> PQYEY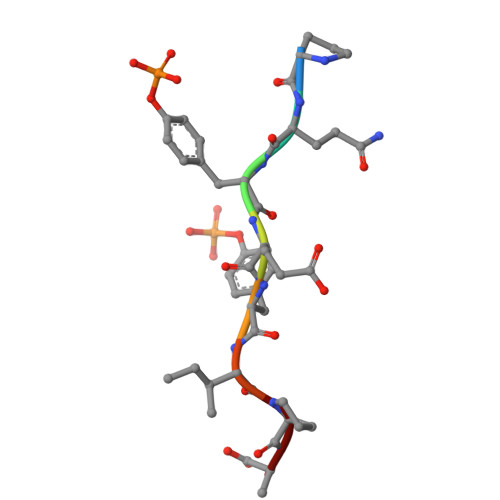IPA>VPTLQRDVAIVGAGPSGLAAATALRKAGLSVAVIEARDRVGGRTWTDTIDGAVLEIGGQWVSPDQTA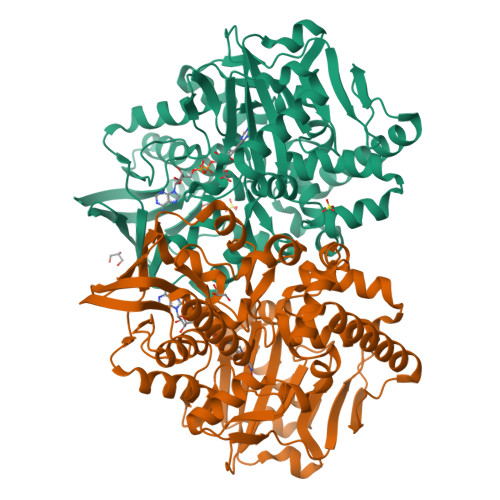LISLLDELGLKTFERYREGESVYISSAGERTRYTGDSFPTNETTKKEMDRLIDEMDDLAAQIGAEEPWAHPLARDLDTVSFKQWLINQSDDAEARDNIGLFIAGGMLTKPAHSFSALQAVLMAASAGSFSHLVDEDFILDKRVIGGMQQVSIRMAEALGDDVFLNAPVRTVKWNESGATVLADGDIRVEASRVILAVPPNLYSRISYDPPLPRRQHQMHQHQSLGLVIKVHAVYETPFWREDGLSGTGFGASEVVQEVYDNTNHEDDRGTLVAFVSDEKADAMFELSAEERKATILASLARYLGPKAEEPVVYYESDWGSEEWTRGAYAASFDLGGLHRYGADSRTPVGPIHFSCSDIAAEGYQHVDGAVRMGQRTAADIIARSKA[2x]3-[(Z)-2-isocyanoethenyl]-1H-indole 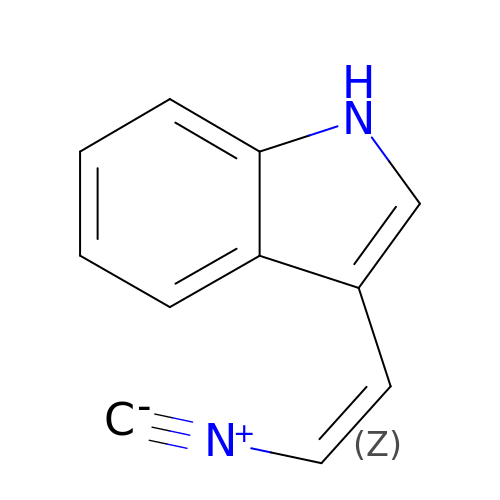| C11 H8 N2 | JQMYMZZLIOIXEO-SREVYHEPSA-N>GAMGNKEKADQQKAVTDIVALENALDMYKLDNSVYPTTDQGLEALVTKPTNPEPRNYREGGYIKRLPKDPW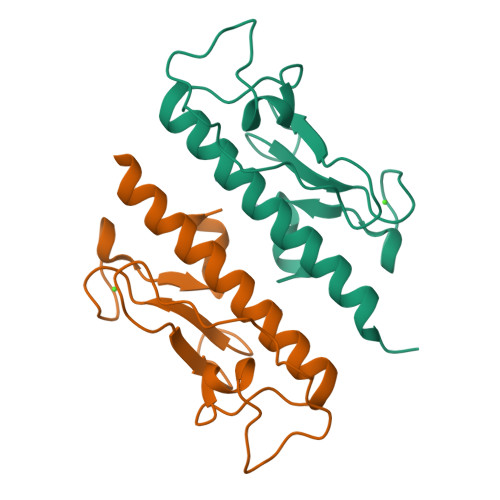GNDYQYLSPGDKGTIDVFTLGADGQEGGEGTGADIGNWNIQDFQ[2x]>[2x]MISLADLQRRIETGELSPNAAIAQSHAAIEAREKEVHAFVRHDKSARAQASGPLRGIAVGIKDIIDTANMPTEMGSEIYRGWQPRSD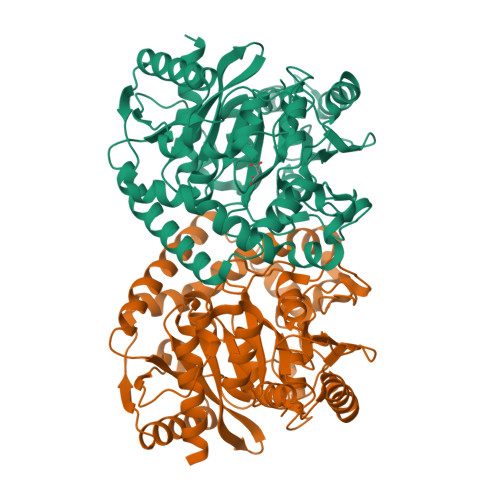APVVMMLKRAGATIIGKTTTTAFASRDPTATLNPHNTGHSPGGSSAGSAAAVGAGMIPLALGTQTGGSVIRPAAYCGTAAIKPSFRMLPTVGVKCYSWALDTVGLFGARAEDLARGLLAMTGRSEFSGIVPAKAPRIGVVRQEFAGAVEPAAEQGLQAAIKAAERAGASVQAIDLPEAVHEAWRIHPIIQDFEAHRALAWEFSEHHDEIAPMLRASLDATVGLTPKEYDEARRIGRRGRRELGEVFEGVDVLLTYSAPGTAPAKALASTGDPRYNRLWTLMGNPCVNVPVLKVGGLPIGVQVIARFGNDAHALATAWFLEDALAKSG> MSLSAHEIRELFLSFFEKKGHTRVKSAPLVPENDPTLLFVNAGMVPFKNVFLGLEKRPYKRATSCQKCLRVSGKHNDLEQVGYTSRHHTFFEMLGNFSFGDYFKKEAIEYAWEFVTEVLKLPKEKLYVSVYKDDEEAYRIWNEHIGIPSERIWRLGEEDNFWQMGDVGPCGPSSEIYVDRGEEYEGDERYLEIWNLVFMQYNRDENGVLTPLPHPNIDTGMGLERIASVLQGKNSNFEIDIIFPLIQFGEEVSGKKYGEKFETDVALRVIADHLRAITFAISDGVIPSNEGRGYVIRRILRRAMRFGYKLGIENPFLYKGVDLVVDIMKEPYPELELSREFVKGIVKGEEKRFIKTLKAGMEYIQEVIQKALEEGRKTLSGKEVFTAYDTYGFPVDLIDEIAREKGLGIDLE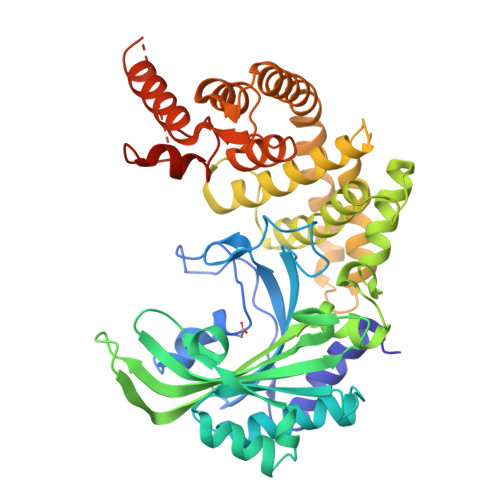GFQCELEEQRERARKHFKVEAKKVKPVYSHLKELGKTSAFVGAAALEHHHHHH> MDWKGRDVISIRDFSKEDIETVLATAERLERELKEKGQLEYAKGKILATLFFEPSTRTRLSFESAMHRLGGAVIGF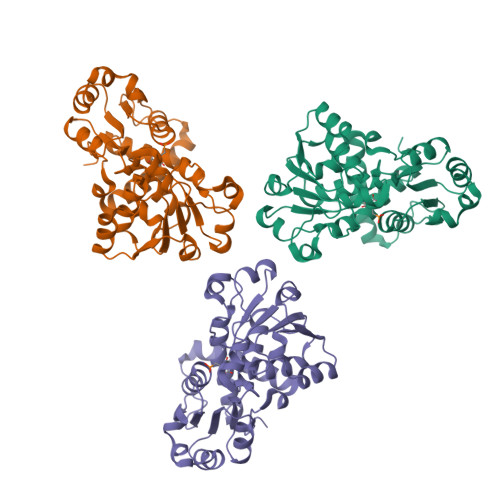AEASTSSVKKGESLRDTIKTVEQYCDVIVIRHPKEGAARLAAEVAEVPVINAGDGSNQHPTQTLLDLYTIKKEFGRIDGLKIGLLGDLKYGRTVHSLAEALTFYDVELYLISPELLRMPRHIVEELREKGMKVVETTTLEDVIGKLDVLYVTRIQKERFPDEQEYLKVKGSYQVNLKVLEKAKDELRIMHPLPRVDEIHPEVDNTKHAIYFRQVFNGVPVRMALLALVLGVI> GSGAMRIGMVCPYSFDVPGGVQSHVLQLAEVLRDAGHEVSVLAPASPHVKLPDYVVSGGKAVPIPYNGSVARLRFGPATHRKVKKWIAEG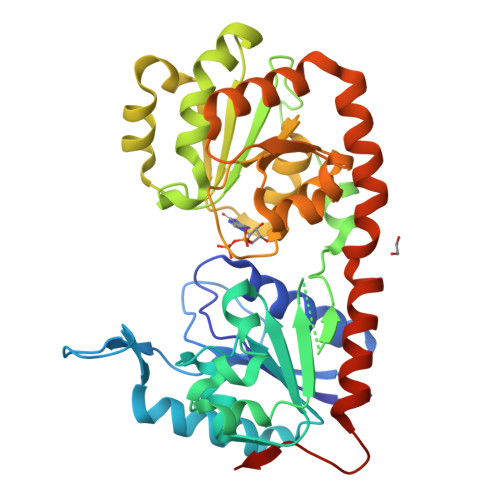DFDVLHIHEPNAPSLSMLALQAAEGPIVATFHTSTTKSLTLSVFQGILRPYHEKIIGRIAVSDLARRWQMEALGSDAVEIPNGVDVASFADAPLLDGYPREGRTVLFLGRYDEPRKGMAVLLAALPKLVARFPDVEILIVGRGDEDELREQAGDLAGHLRFLGQVDDATKASAMRSADVYCAPHLGGESFGIVLVEAMAAGTAVVASDLDAFRRVLADGDAGRLVPVDDADGMAAALIGILEDDQLRAGYVARASERVHRYDWSVVSAQIMRVYETVSGAGIKVQVSGAANRDETAGESV>[2x]MNSELDYYEKFEEVHGILMYKDFVKYWDNVEAFQARPDDLVIATYPKSGTTWVSEIVYMIYKEGDVEKCKEDVIFNRIPFLECRKENLMNGVKQLDEMNSPRIVKTHLPPELLPASFWEKDCKIIYLCRNAKDVAVSFYYFFLMVAGHPNPGSFPEFVEKFMQGQVPYGSWYKHVKSWWEKGKSPRVLFLFYEDLKEDIRKEVIKLIHFLERKPSEELVDRIIHHTSFQEMKNNPSTNYTTLPDEIMNQKLSPFMRKGITGDWKNHFTEALNEKFDKHYEQQMKESTLKFRTEI

In humans, there are 13 cytosolic sulfotransferases that catalyze the transfer of a sulfuryl group (SO3) from the donor cofactor 3´-phosphate 5´-phosphosulfate (PAPS) to acceptor substrates, including xenobiotics, fatty acids, neurotransmitters, and steroids. Sulfation of 17β-estradiol (E2) by human estrogen sulfotransferase (SULT1E1) results in loss of binding to the estrogen receptor as well as increased availability for renal excretion, thereby effectively regulating the concentration of E2. To understand the binding and inhibition of estrogen sulfotransferase by BFRs, we obtained crystal structures of SULT1E1 in complex with the product cofactor PAP and three different compounds bound at the active site: the natural substrate (E2), a BFR (TBBPA), and a human BFR metabolite (3-OH-BDE-47) at resolutions of 1.95 Å, 2.0 Å, and 2.05 Å, respectively. SULT1E1 crystallizes with two molecules in the asymmetric unit (designated molecule A and molecule B) representing the proposed physiological dimer.

The co-crystal structure of PAP and TBBPA bound to SULT1E1 reveals TBBPA binding in the same substrate binding pocket as E2. In molecule B, the position of the TBBPA is well determined because there is clear electron density for the entire molecule, with strong density for the first phenolic ring and slightly weaker density for the second ring, suggesting that this ring contains greater conformational flexibility. The first phenolic ring of TBBPA superimposes with the phenolic ring of E2, positioning the 4-hydroxyl within hydrogen bonding distance to the catalytic base His107, similar to the 3-hydroxyl of E2. In addition, this ring neatly fits between the steric gate residues Phe80 and Phe141. The second ring is located out of the plane with respect to E2 and extends into a different region of the hydrophobic binding pocket. The bromine (Br5) bound to the C5 carbon is buried in a hydrophobic cavity within van der Waal distance (4.3 Å) of Tyr20, Phe80, His107, Phe141, and Tyr168. Bromine atom Br3 is located in a more hydrophilic environment and is potentially able to form hydrogen or halogen bonds with Lys105 (3.1 Å) and/or Tyr239 (3.2 Å). Overall, the protein conformation of SULT1E1 with bound TBBPA is very similar to that with bound E2 with only a few minor changes in the substrate binding pocket. Binding of TBBPA results in increased sidechain order for Met247, whereas the sidechain of Ile246 becomes slightly more disordered and the conformation of loop residues 84–89 is altered (2.0 Å shift at Cα atom of Asn87 in molecule B). Although the electron density for TBBPA in molecule A is not as clear for the second ring, it appears that the overall position of the molecule is slightly shifted with respect to the position in molecule B. This shift is correlated with a shift in the loop (4.5 Å at Cα atom of Asn87 in molecule A compared with molecule B of the E2-bound structure) containing residues 84–89.> GKQRILLYLVNKLNNIYFRIESPQLCSNIFKNFQPKSMLAHF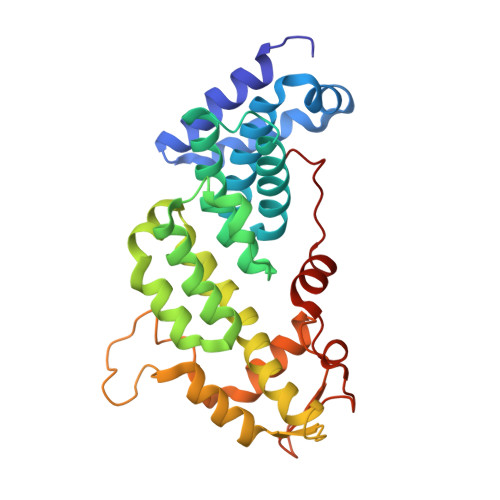NEYQLDQQIEYRYLLGRYYLLNSQVHNAFVQFNEAFQSLLNLPLTNQAITRNGTRILNYMIPTGLILGKMVKWGPLRPFLSQETIDNWSVLYKHVRYGNIQGVSLWLRQNERHLCARQLLIVLLEKLPMVTYRNLIKTVIKSWTTEWGQNKLPYSLIERVLQLSIGPTFEDPGAQEITIYNGIHSPKNVENVLVTLINLGLLRANCFPQLQLCVVKKTTMIQEIVPPVNERITKMFPAHSHVLW>APAAVDWRARGAVTAVKDQGQ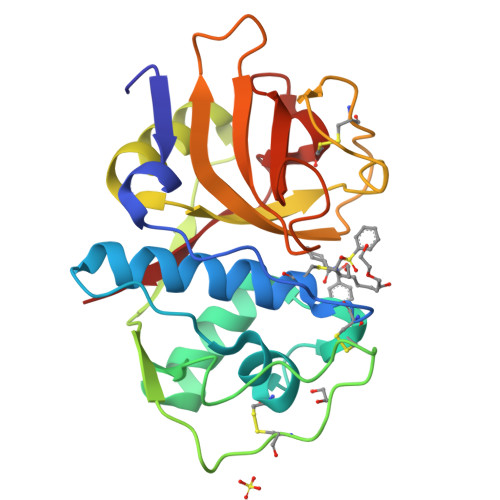CGSCWAFSAIGNVECQWFLAGHPLTNLAEQMLVSCDKTDSGCSGGLMNNAFEWIVQENNGAVYTEDSYPYASGEGISPPCTTSGHTVGATITGHVELPQDEAQIAAWLAVNGPVAVAVDASSWMTYTGGVMTSCVSEQLDHGVLLVGYNDGAAVPYWIIKNSWTTQWGEEGYIRIAKGSNQCLVKEEASSAVVG[2x]>[4x]YRPISQGVSDLVGLPNQICLQKTTSTILKPRLISYTLPINTREGVCITDPLLAVDNGFFAYSHLEKIGSCTRGIAKQRIIGVGEVLDRGDKVPSMFMTNVWTPPNPSTIHHCSSTYHEDFYYTLCAVSHVGDPILNSTSWTESLSLIRLAVRPKSDSGDYNQKYIAITKVERGKYDKVMPYGPSGIKQGDTLYFPAVGFLPRTEFQYNDSNCPIIHCKYSKAENCRLSMGVNSKSHYILRSGLLKYNLSLGGDIILQFIEIADNRLTIGSPSKIYNSLGQPVFYQASYSWDTMIKLGDVDTVDPLRVQWRNNSVISRPGQSQCPRFNVCPEVCWEGTYNDAFLIDRLNWVSAGVYLNSNQTAENPVFAVFKDNEILYQVPLAEDDTNAQKTITDCFLLENVIWCISLVEIYDTGDSVIRPKLFAVKIPAQCSESGRGLVPR;>SIVLEPIYWNSSNSKFLPGQGLVLYPQIGDKLDIICPKVDSKTVGQYEYYKVYMVDKDQADRCTIKKENTPLLNCAKPDQDIKFTIKFQEFSPNLWGLEFQKNKDYYIISTSNGSLEGLDNQEGGVCQTRAMKILMKVGQD[4x]

The henipaviruses possess an attachment (G) and a fusion (F) glycoprotein which together work in concert to mediate the virus attachment and entry process, but the precise triggering mechanism of paramyxovirus fusion has yet to be defined in detail. The henipavirus G glycoproteins have a type-II transmembrane topology, containing a short N-terminal cytoplasmic tail and a long C-terminal extracellular globular head. Distinct from most other members within the subfamily Paramyxovirinae, the henipavirus attachment glycoprotein does not hemagglutinate and neither binds to sialic acid, nor retains neuraminidase activity, and instead binds cell surface protein receptors. Recently, ephrin-B2 and ephrin-B3 were identified as the functional receptors for both HeV and NiV.

The high-resolution structures described here, including both HeV-G alone (2.2 Å) and in complex with ephrin-B2 (2.7 Å), combined with structure-based mutagenesis, reveal new insights into the molecular mechanisms governing the initial steps of henipavirus entry into host cells and into the paramyxovirus entry mechanism in general. HeV-G and ephrin-B2 form 1∶1 complex both in solution and in the crystals. Four copies of complex were observed in the asymmetric unit of the crystal. The complex buries an interface of 1272 Å2, slightly smaller than the 1354 Å2 buried in the NiV-G/ephrin-B3 complex and the 1393 Å2 - in NiV-G/ephrin-B2 complex. Ephrin-B2 (S27-D167) used in our structural studies here was expressed in stably-transfected human HEK293 cells. Thus, its glycosylation pattern is more physiologically relevant than in the previously published structures, which used ephrin expressed in either yeast, bacteria or in the presence of glycosylation inhibitor. In addition to the previously observed glycosylation site N36, we now observe another glycosylation site - N139, which is consistent with sequence-based predictions. Ephrin-B2 undergoes very minor conformational changes upon binding to HeV-G and its structure in the HeV-G/ephrin-B2 complex can be superimposed on the unbound ephrin-B2 structure with the root mean square deviation (RMSD) between equivalent Cα positions of approximately 0.5 Å. The only region on ephrin-B2 that shows some rearrangements upon HeV-G binding is the G-H loop. These conformational changes within this ephrin region are necessary to fit its four hydrophobic residues (F, P, L and W) within the G-H loop into their binding pockets on the HeV-G surface.> MRGSAHVVILGAGTGGMPAAYEMKEALGSGHEVTLISANDYFQFVPSNPWVGVGWKERDDIAFPIRHYVERKGIHFIAQSAEQIDAEAQNITLADGNTVHYDYLMIATGPKLAFENVPGSDPHEGPVQAICTVDHAERAFAEYQALLREPGPIVIGAMAGASCFGPAYEYAMIVASDLKKRGMRDKIPSFTFITSEPYIGHLGIQGVGDSKGILTKGLKEEGIEAYTNCKVTKVEDNKMYVTQVDEKGETIKEMVLPVKFGMMIPAFKGVPAVAGVEGLCNPGGFVLVDEHQRSKKYANIFAAGIAIAI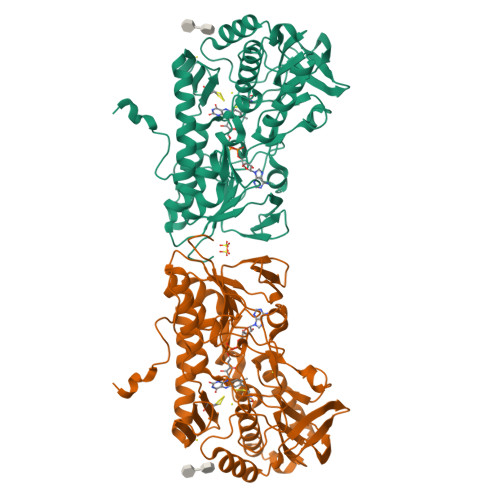PPVETTPVPTGAPKTGYMIESMVSAAVHNIKADLEGRKGEQTMGTWNAVCFADMGDRGAAFIALPQLKPRKVDVFAYGRWVHLAKVAFEKYFIRKMKMGVSEPFYEKVLFKMMGITRLKEEDTHRKAS>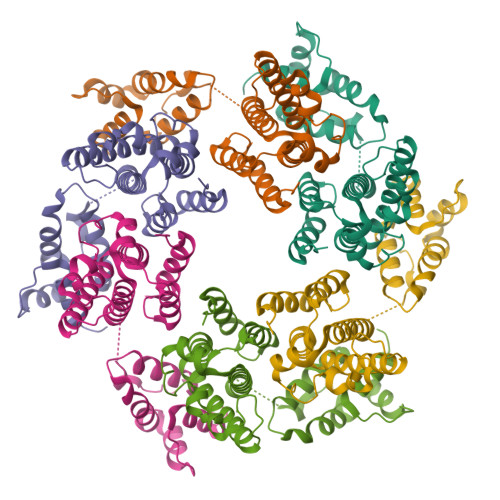[6x]PVVIKTEGPAWTPLEPKLITRLADTVRTKGLRSPITMAEVEALMSSPLLPHDVTNLMRVILGPAPYALWMDAWGVQLQTVIAAATRDPRHPANGQGRGERTNLNRLKGLADGMVGNPQGQAALLRPGELVAITASALQAFREVARLAEPAGPWADIMQGPSESFVDFANRLIKAVEGSDLPPSARAPVIIDCFRQKSQPDIQQLIRTAPSTLTTPGEIIKYVLDRQKTA>[2x]MDSGPKVVIDGKDQNV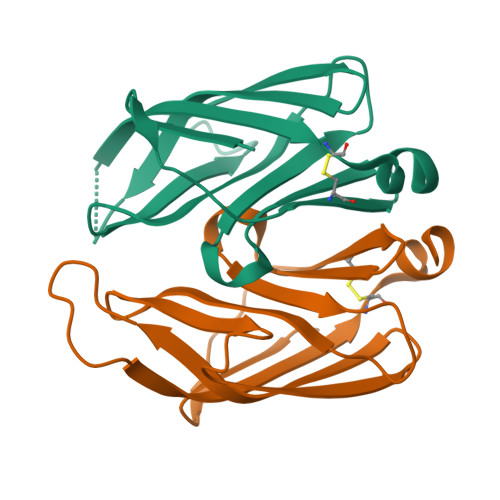TGSVVCTTAAGNVNIAIGGAATGIAAVLTDGNPPEVKSVGLGNVNGVTLGYTSGTGQGNASATKDGSHYKITGTATGVDMANPMSPVNKSFEIEVTCSTKLAAALEHHHHHH>[4x]MGNRGMEDLIPLVNRLQDAFSAIGQNADLDLPQIAVVGGQSAGKSSVLENFVGRDFLPRGSGIVTRRPLVLQLVNATTEYAEFLHCKGKKFTDFEEVRLEIEAETDRVTGTNKGISPVPINLRVYSPHVLNLTLVDLPGMTKVPVGDQPPDIEFQIRDMLMQFVTKENCLILAVSPANSDLANSDALKVAKEVDPQGQRTIGVITKLDLMDEGTDARDVLENKLLPLRRGYIGVVNRSQKDIDGKKDITAALAAERKFFLSHPSYRHLADRMGTPYLQKVLNQQLTNHIRDTLPGLRNKLQSQLLSIEKEVEEYKNFRPDDPARKTKALLQMVQQFAVDFEKRIEGSGDQIDTYELSGGARINRIFHERFPFELVKMEFDEKELRREISYAIKNIHGIRTGLFTPDMAFETIVKKQVKKIREPCLKCVDMVISELISTVRQCTKKLQQYPRLREEMERIVTTHIREREGRTKEQVMLLIDIELAYMNTNHEDFIGFANAQQRSNQMNKKKTSGNQDEILVIRKGWLTINNIGIMKGGSKEYWFVLTAENLSWYKDDEEKEKKYMLSVDNLKLRDVEKGFMSSKHIFALFNTEQRNVYKDYRQLELACETQEEVDSWKASFLRAGV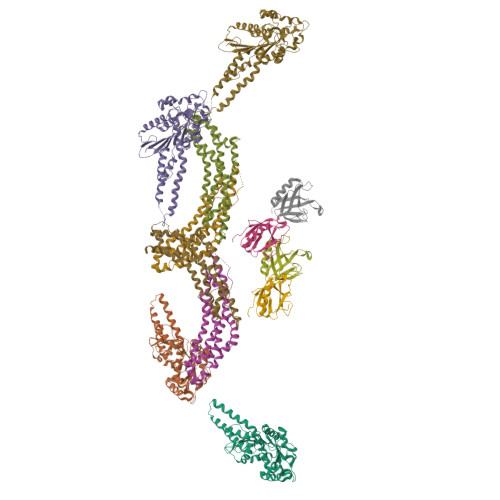YPERVGDKEKASETEENGSDSFMHSMDPQLERQVETIRNLVDSYMAIVNKTVRDLMPKTIMHLMINNTKEFIFSELLANLYSCGDQNTLMEESAEQAQRRDEMLRMYHALKEALSIIGNINTTTVSTPMPPPVDDSWLQVQSVPAGRRSPTSSPTPQRRAPAVPPARPGSRGPAPGPPPAGSALGGAPPVPSRPGASPDPFGPPPQVPSRPNRAPPGVPSRSGQASPSRPESPRPPFDL;>MGNRGMEDLIPLVNRLQDAFSAIGQNADLDLPQIAVVGGQSAGKSSVLENFVGRDFLPRGSGIVTRRPLVLQLVNATTEYAEFLHCKGKKFTDFEEVRLEIEAETDRVTGTNKGISPVPINLRVYSPHVLNLTLVDLPGMTKVPVGDQPPDIEFQIRDMLMQFVTKENCLILAVSPANSDLANSDALKVAKEVDPQGQRTIGVITKLDLMDEGTDARDVLENKLLPLRRGYIGVVNRSQKDIDGKKDITAALAAERKFFLSHPSYRHLADRMGTPYLQKVLNQQLTNHIRDTLPGLRNKLQSQLLSIEKEVEEYKNFRPDDPARKTKALLQMVQQFAVDFEKRIEGSGDQIDTYELSGGARINRIFHERFPFELVKMEFDEKELRREISYAIKNIHGIRTGLFTPDMAFETIVKKQVKKIREPCLKCVDMVISELISTVRQCTKKLQQYPRLREEMERIVTTHIREREGRTKEQVMLLIDIELAYMNTNHEDFIGFANAQQRSNQMNKKKTSGNQDEILVIRKGWLTINNIGIMKGGSKEYWFVLTAENLSWYKDDEEKEKKYMLSVDNLKLRDVEKGFMSSKHIFALFNTEQRNVYKDYRQLELACETQEEVDSWKASFLRAGVYPERVGDKEKASETEENGSDSFMHSMDPQLERQVETIRNLVDSYMAIVNKTVRDLMPKTIMHLMINNTKEFIFSELLANLYSCGDQNTLMEESAEQAQRRDEMLRMYHALKEALSIIGDINTTTVSTPMPPPVDDSWLQVQSVPAGRRSPTSSPTPQRRAPAVPPARPGSRGPAPGPPPAGSALGGAPPVPSRPGASPDPFGPPPQVPSRPNRAPPGVPSRSGQASPSRPESPRPPFDL[8x]> MGSDKIHHHHHHMTVLIIGMGNIGKKLVELGNFEKIYAYDRISKDIPGVVRLDEFQVPSDVSTVVECASPEAVKEYSLQILKNPVNYIIISTSAFADEVFRERFFSELKNSPARVFFPSGAIGGLDVLS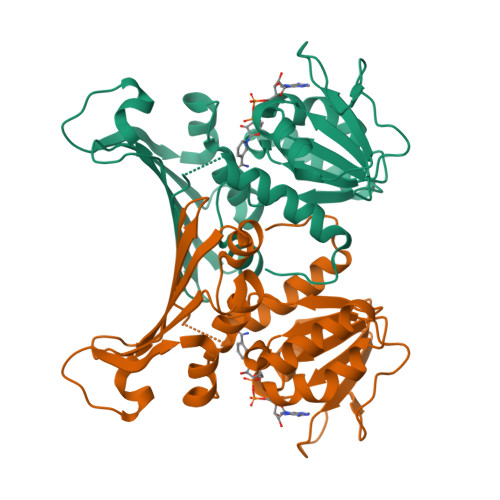SIKDFVKNVRIETIKPPKSLGLDLKGKTVVFEGSVEEASKLFPRNINVASTIGLIVGFEKVKVTIVADPAMDHNIHIVRISSAIGNYEFKIENIPSPENPKTSMLTVYSILRTLRNLESKIIFG> GRLL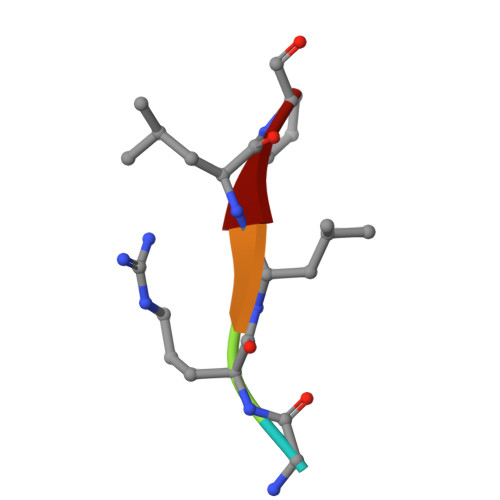P>[2x]ANIVGGIEYSINNASLCSVGFSVTRGATKGFVTAGHCGTVNAT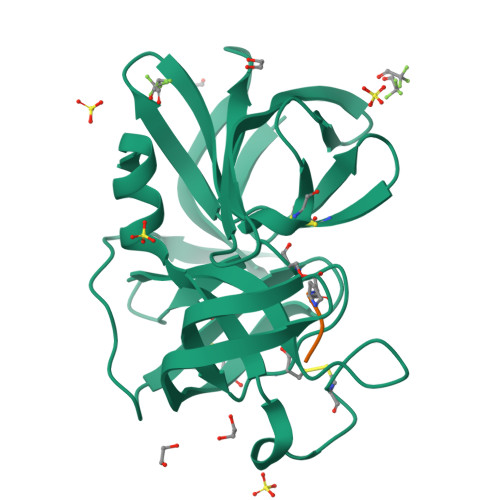ARIGGAVVGTFAARVFPGNDRAWVSLTSAQTLLPRVANGSSFVTVRGSTEAAVGAAVCRSGRTTGYQCGTITAKNVTANYAEGAVRGLTQGNACMGRGDSGGSWITSAGQAQGVMSGGNVQSNGNNCGIPASQRSSLFERLQPILSQYGLSLVTG>[2x]MGEIESYCNKELGPLPTKAPTLSKNVLDLFSLKGKVASVTGSSGGIGWAVAEAYAQAGADVAIWYNSHPADEKAEHLQKTYGVHSKAYKCNISDPKSVEETISQQEKDFGTIDVFVANAGV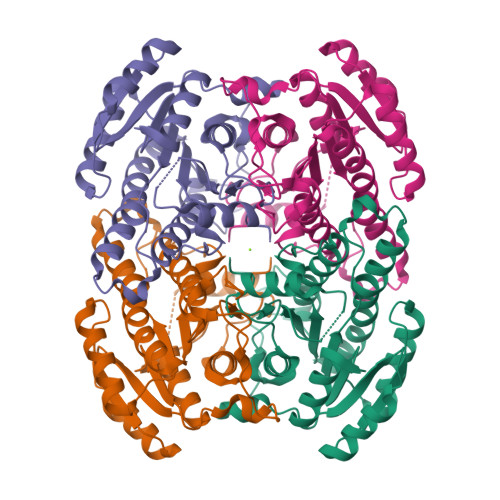TWTQGPEIDVDNYDSWNKIISVDLNGVYYCSHNIGKIFKKNGKGSLIITSSISGKIVNIPQLQAPYNTAKAACTHLAKSLAIEWAPFARVNTISPGYIDTDITDFASKDMKAKWWQLTPLGREGLTQELVGGYLYLASNASTFTTGSDVVIDGGYTCP> ASRHLRFENLTEEQLKRLAKILTENLKGGEVVILSGNLGAGKTTFVKGMIRAIGLDEKMVKSPTFTLMNVYPGLKTIYHLDLYRLQDTDFLSLDVEDILEDEDGIMVVEWGDLFDGFWP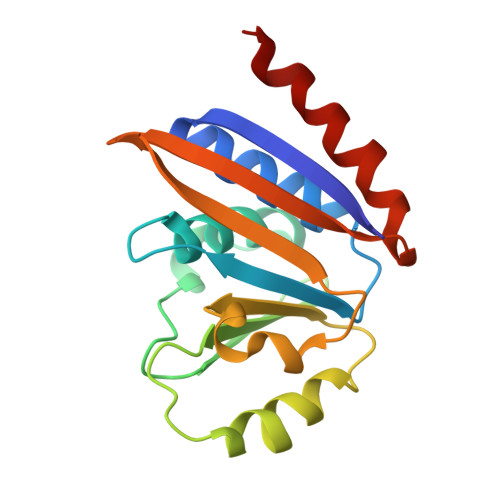EDSIKVKIEIADESHRNVEILIPEEVNFLVEKIERYRKELQNT> CCCCGGG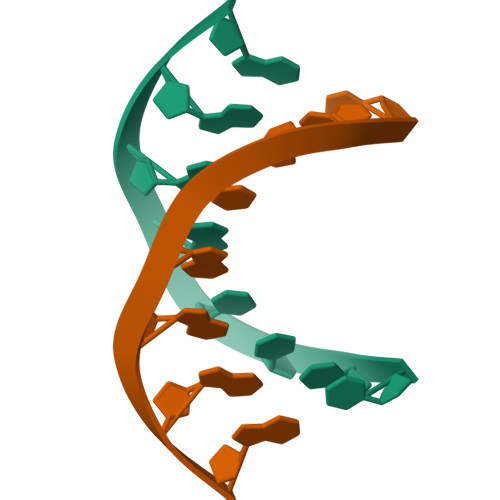G>ANLERTFIAIKPDGVQRGLVGEIIKRFEQKGFRLVAMKFLRASEEHLKQHYIDLKDRPFFPGLVKYMNSGPVVAMVWEGLNVVKTGRVMLGETNPADSKPGTIRGDFCIQVGRNIIHGSDSVKSAEKEISLWFKPEELV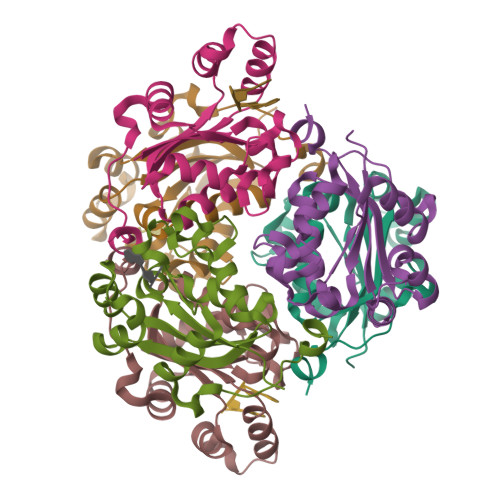DYKSCAHDWVYE[6x]> PEKRVAS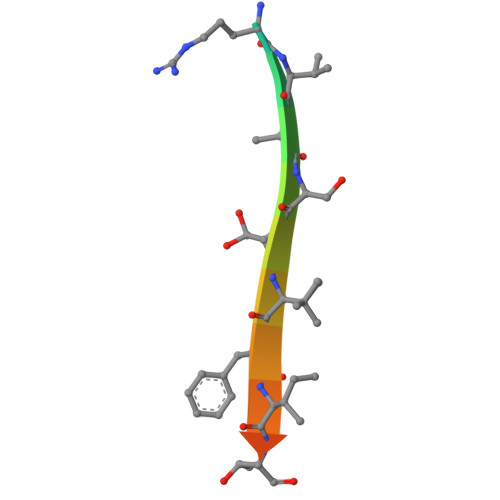SVFITLAP>[4x]AECSVDIQGNDQMQFNTNAITVDKSCKQFTVNLSHPGNLPKNVMGHNWVLSTAADMQGVVTDGMASGLDKDYLKPDDSRVIAHTKLIGSGEKDSVTFDVSKLKEGEQYMF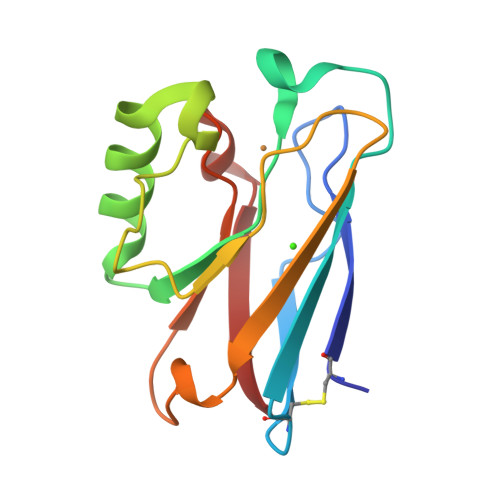FCTFPGHSALMKGTLTLK> MSATTTNLKEAIVNRRSIRKVTKNDAITKERIEEVLKTALHAPTSFNMQSGRMVVLMDGEHEKFWDIVKE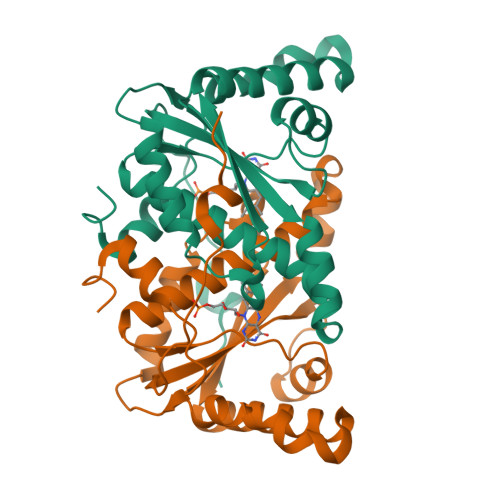TLRARVPAENFEATVERLKGFHAGVGTVLFFEDQATVEKMQENAPLYKDQFPFWSHQGNAMLQHTVWMLLSAEGIGASLQHYNPIVDAEVKETWNIPAEWSLVGQMPFGEPNEQPAERTFLPTEDVVKFY>GPLGSDADKNDPAGKDQQVNVGETPKAEDSIGNLPDLPKGTTVAFETPVD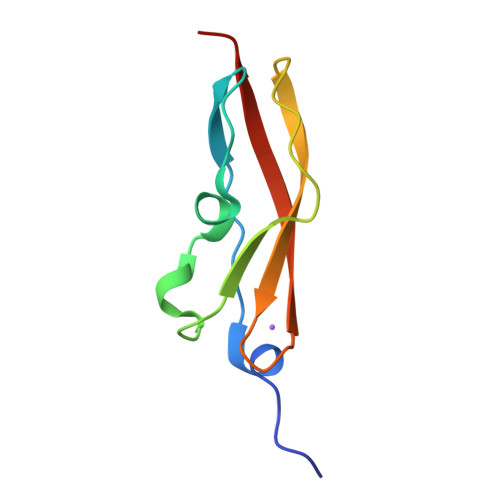TATPGDKPAKVVVTYPDGSKDTVDVTVKVVDPRT[2x]> MAAPQFHRPSTITADNVRALGMRGLVLATNNAQFIMDNSY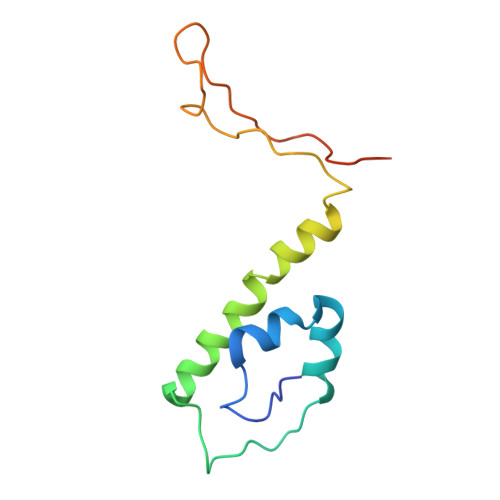PHPHGTQGAVREFLRGQAAALTDLGVTHANNTFAPQPMFAGDAAAEWLRPSFGLKRTYSPFVVRDPKTPSTP> MDTAGDTKSGSDGGVVNITYMHRLPDSKGMTLVNDIVAKWNKEHPNIQVKATKFDGKASEMIKKLETDVKAGNAPDLAQVGYAEVPEVFTKGLLQDVTDEAAKYKDDFASAPFALMQVDGKTYGLPQDTGPLAYFYNAAEFEKLGITVPKTADELIETAKKTAAQGKYIMTFQPDEAMMMMSGQAGASGPWYKVDGNSWVVNTQTKGSKAVADVYQQLIDNKAALTNPRWDASFD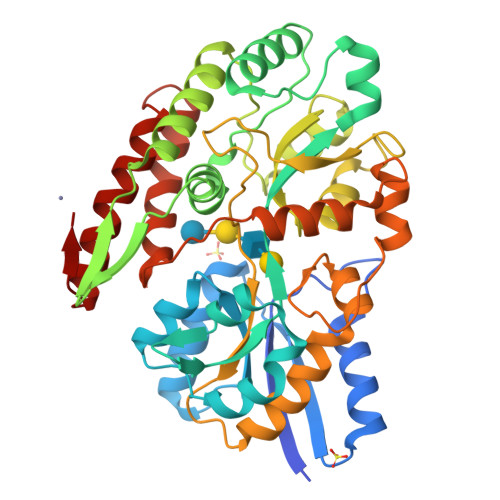NSIQSGQLIGTVAAAWEAPLFIDSAGGTGAGEWKVTQLGDWFGNGTKTGSDGGSGVAVLKGSKHPAEAMEFLDWFNTQVDDLVSQGLVVAATTADAKTPQKWSDYFSGQDVMAEFKTANDNMGDFTYMPGFSAVGAAMKQTAAKAADGSAKVSDVFDTAQKTSVDTLKNLGLSVKE1-(2-piperazin-1-ylethyl)-5-pyridin-4-yl-indole | 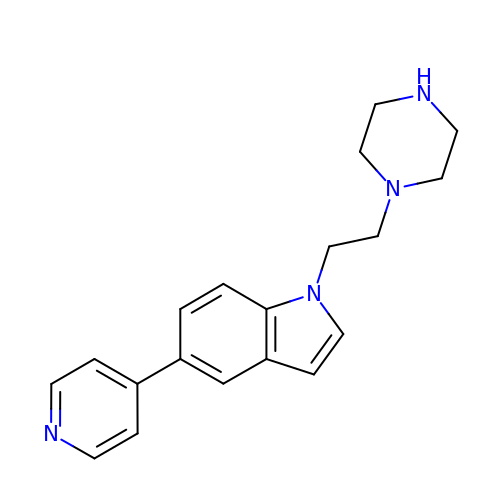C19 H22 N4 | VBMJJJLARMSVGX-UHFFFAOYSA-N CPS secretion is mediated by an ABC transporter containing KpsT and KpsM as its nucleotide-binding domain (NBD) and transmembrane domain, respectively. The transporter partners with the periplasmic and inner-membrane-anchored KpsE subunit, a class-3 polysaccharide co-polymerase (PCP), as well as with KpsD, which is assumed to form an outer-membrane pore. The KpsMT transporter is surrounded by a cage of eight KpsE subunits extending about 80 Å into the periplasm. Cryo-electron microscopy analyses of the KpsMT–KpsE complex in six different states reveal a KpsE-encaged ABC transporter, rigid-body conformational rearrangements of KpsMT during ATP hydrolysis and recognition of a glycolipid inside a membrane-exposed electropositive canyon.

To determine how KpsMT recognizes the glycolipid, the purified KpsMT–KpsE complex was preincubated with the isolated glycolipid before cryo grid preparation. Cryo-EM analyses of this sample provided additional cryo-EM maps similar in overall architecture to the Apo 1 state, but with poorly defined KpsT subunits. KpsT was therefore placed after focused refinement and rigid-body docking. However, in contrast to all other structures, we identified two states of a lipid molecule bound inside the canyon (referred to as state-1 and state-2). In state-2, the lipid is shifted by about 7 Å towards the periplasm, such that the carboxyl group of the putative Kdo sugar is in proximity to Arg35 and Arg94 of the interface helix and TM2, respectively. The lipid phosphate group contacts Arg187 of TM5 in the opposing KpsM subunit. Furthermore, at the C-terminal end of this helix, Gln181 is suitably positioned to interact with the Kdo moiety. Relative to the estimated cytosolic and periplasmic membrane boundaries, the glycolipid sits about halfway across the membrane, in agreement with it representing a translocation substrate. Compared with state-1, the second lipid-binding pose further correlates with an approximately 6 Å rigid-body translation of the KpsM subunits against each other, thereby widening the space between the KpsM protomers and narrowing the entry to the polysaccharide canyon by around 3 Å. Extending this KpsM movement could create a channel-forming transporter conformation, as observed for the O-antigen WzmWzt transporter.

>[2x]MIELRNLTKWYPTPHGRRYVFRNLNFRFPDDVSIGLIGRNGAGKSTLMRLLGGIEAPNEGEVVTDVSISWPVGLSGGFQGSLTARENVKFVCRIYGTSHEDMLRKVRFVEEFAEIGEHFDLPMKTYSSGMRSRVAFGLSMAFDFDYYLIDEAMAVGDAQFRAKSRAVFDSRVGQANMILVSHNMNDIKEYCDVVVLVDQGQATLYEDVEAGIAAYQGSLKKAAAKPDYKDDDDK;>MGKIHLAVSERSPRVKRSPWQIQQAVLFALFLRELKTRLGGRWLGVFWVLLEPVAHIAVMTTLFSLAHRAAMPSIEYPVFLITGLIPFFMFRGLVTRLMEAIDSNRGLFAYRQVKPIDTVIARAMLEISLQSIVYLIALGTLGWLGFHFLPVRALELAGVSAVLIMLGASLGLFFAVVTNEIPQARAIVRISLLPLYFVSGVIFPVHTIPPQYLPLLQLNPVLHLIELSRASFFPQYRVLQGINLAYPAGFALLSLFLALMLYRLRRHQLASVV[2x];>[8x]MGKIHMKLVSRLTAKRLQWALVYLPMLVATVYFLVFSADRYVSESVITVRQTSSNAPTGGMSGAALLLAGLTPASREDTCYLQTYIHSMGLLQKLDQQLKLREHFGTPLRDPLFRLWGGTSQEWFLEYYRSRVEVLMDDICGLLTVRVQGFEPEFAQALNRAILEESERFVNELSHRMAREQGQFAEAELERATARLQEAKRQLIAFQAKHKLLDPLAQAQATGTLTAELQAALTRQEAELRNALTYLNEDSYQVKALRSQINALRQQIDEERLRATAGKNGDRINAVAAEFHDLQLQVGFAEDAYKLALAAVESARIEATRKLKSLVVVEPPVLPEIAEYPRRWYNLATLLVVCCLIYGVVSLVVATIRDHQDGSGSGSHHHHHHHHHH> AEIKAVSAARLLDVASGKYVDNPLVIV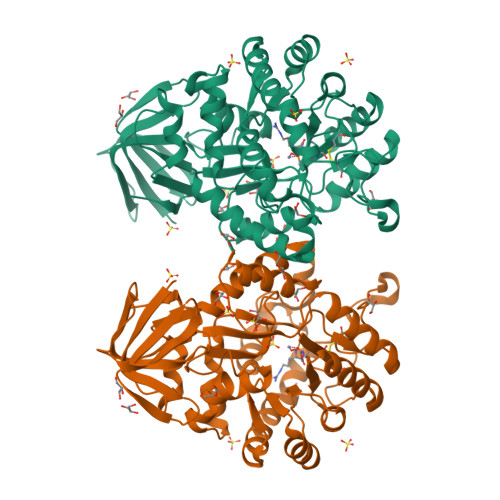TDGRITSIGKKGDAVPAGATAVDLPGVTLLPGLIDMHVHLDSLAEVGGYNSLEYSDRFWSVVQTANAKKTLEAGFTTVRNVGAADYDDVGLREAIDAGYVPGPRIVTAAISFGATGGHCDSTFFPPSMDQKNPFNSDSPDEARKAVRTLKKYGAQVIKICATGGVFSRGNEPGQQQLTYEEMKAVVDEAHMAGIKVAAHAHGASGIREAVRAGVDTIEHASLVDDEGIKLAVQKGAYFSMDIYNTDYTQAEGKKNGVLEDNLRKDRDIGELQRENFRKALKAGVKMVYGTDAGIYPHGDNAKQFAVMVRYGATPLQAIQSATLTAAEALGRSKDVGQVAVGRYGDMIAVAGDPLADVTTLEKPVFVMKGGAVVKAP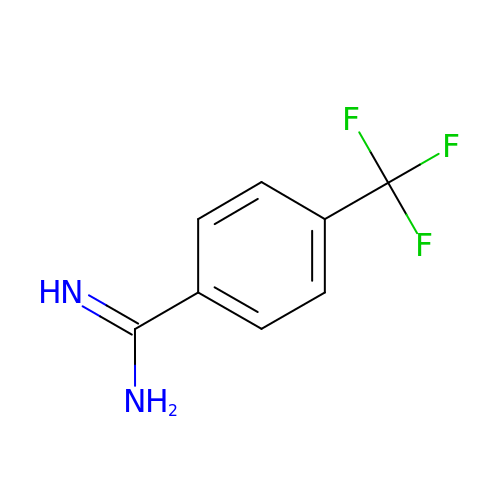4-(trifluoromethyl)benzenecarboximidamide | C8 H7 F3 N2 | XFLGYXVBXUAGQV-UHFFFAOYSA-N> ADLEAVLADVSYLMAMEKSKATPAARASKKILLPEPSIRSVMQKYLEDRGEVTFEKIFSQKLGYLLFRDFCLKHLEEAKPLVEFYEEIKKYEKLETEEERLVCSREIFDTYIMKELLACSHPFSKSAIEHVQGHLVKKQVPPDLFQPYIEEICQNLRGDVFQKFIESDKFTRFCQWKNVELNIHLTMNDFSVHRIIGRGGFGEVYGCRKADTGKMYAMKCLDKKRIKMKQGETLALNERIMLSLVSTGDCPFIVCMSYAFHTPDKLSFILDLMNGGDLHYHLSQHGVFSEPDMIFYAAEIILGLEHMHNRFVVYRDLKPANILLDEHGHVRISDLGLACDFSKKKPHASVGTHGYMAPEVLQKGVAYDSSADWFSLGCMLFKLLRGHSPFRQHKTKDKHEIDRMTLTMAVELPDSFSPELRSLLEGLLQRDVNRRLGCLGRGAQEVKESPFFRDLDWQMVFLQKYPPPLIPPRGEVNAADA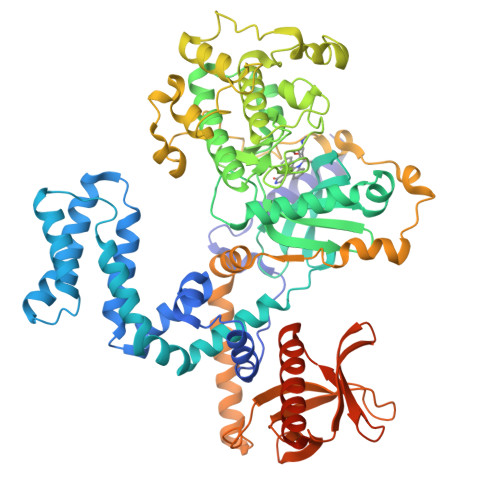FDIGSFDEEDTKGIKLLDSDQELYRNFPLTISERWQQEVAETVFDTINAETDRLEARKKTKNKQLGHEEDYALGKDCIMHGYMSKMGNPFLTQWQRRYFYLFPNRLEWRGEGEAPQSLLTMEEIQSVEETQIKERKCLLLKIRGGKQFVLQCDSDPELVQWKKELRDAYREAQQLVQRVPKMKNKPRSPVVELSKVPLIQRGSANGL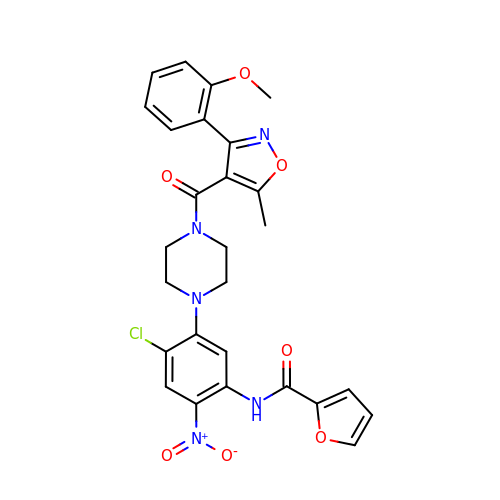N-[4-chloranyl-5-[4-[[3-(2-methoxyphenyl)-5-methyl-1,2-oxazol-4-yl]carbonyl]piperazin-1-yl]-2-nitro-phenyl]furan-2-carboxamide | C27 H24 Cl N5 O7 | SFVFADOVSFCYBD-UHFFFAOYSA-N> EITVDEFSNIRENPVTPWNPEPSAPVIDPTAYIDPQASVIGEVTIGANVMVSPMASIRSDEGMPIFVGDRSNVQDGVVLHALETINEEGEPIEDNIVEVDGKEYAVYIGNNVSLAHQSQVHGPAAVGDDTFIGMQAFVFKSKVGNNCVLEPRSAAIGVTIPD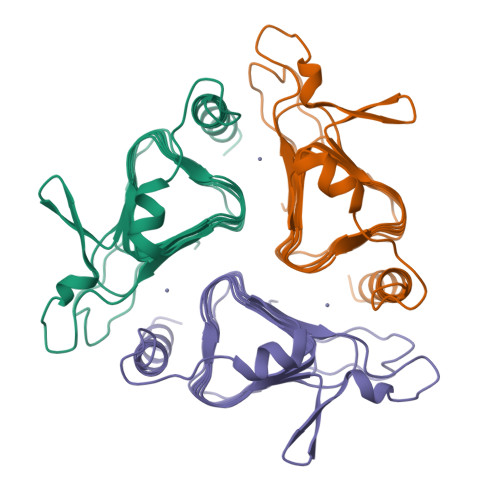GRYIPAGMVVTSQAEADKLPEVTDDYAYSHTNEAVVYVNVHLAEGYKETS> KSVLEDNLPFLEFPGSIVYSYEASDCSFLSEDISMRLSDGDVVGFDMEWPPIYKPGKRSRVAVIQLCVSESKCYLFHISSMSVFPQGLKMLLENKSIKKAGVGIEGDQWKLLRDFDVKLESFVELTDVANEKLKCAETWSLNGLVKH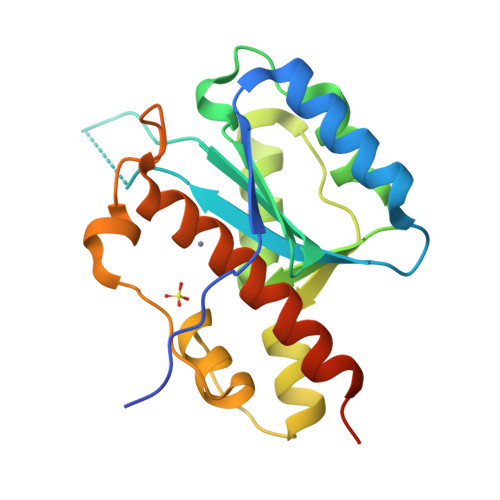VLGKQLLKDKSIRCSNWSNFPLTEDQKLYAATDAYAGLIIYQKLGNLGDTVQVFALNKAEE>[6x]GLSDWELAAARA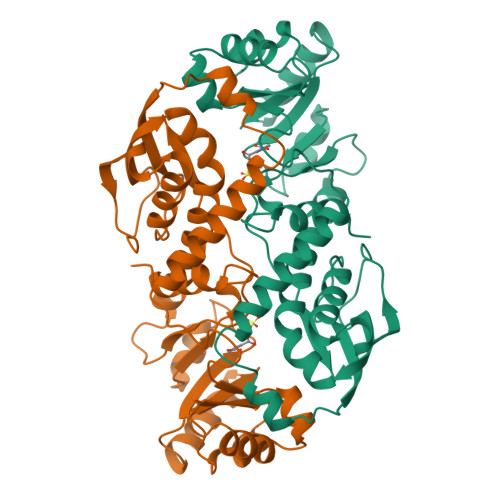AIARGLDEDLRYGPDVTTLATVPASATTTASLVTREAGVVAGLDVALLTLNEVLGTNGYRVLDRVEDGARVPPGEALMTLEAQTRGLLTAERTMLNLVGHLSGIATATAAWVDAVRGTKAKIRDTRKTLPGLRALQKYAVRTGGGVNHRLGLGDAALIKDNHVAAAGSVVDALRAVRNAAPDLPCEVEVDSLEQLDAVLPEKPELILLDNFAVWQTQTAVQRRDSRAPTVMLESSGGLSLQTAATYAETGVDYLAVGALTHSVRVLDIGLDM>[120x]MGNAKTRRRERRAEKQAQWKAANAGAGAGAMATPHFDYIASEVSKGLANLSL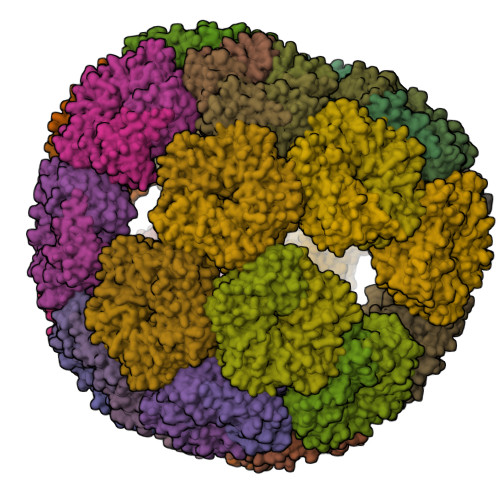ELRKPITFGVITADTLEQAIERAGTKHGNKGWEAALSAIEMANLFKSLRGTGHHHHHHGSSMEIYEGKLTAEGLRFGIVASRFNHALVDRLVEGAIDCIVRHGGREEDITLVRVPGSWEIPVAAGELARKEDIDAVIAIGVLIRG> MAEVLRTLAGKPKCHALRPMILFLIMLVLVLFGYGVLSPRSLMPGSLERGFCMAVREPDHLQRVSLPRMVYPQPKVLTPCRKDVLVVTPWLAPIVWEGTFNIDILNEQFRLQNTTIGLTVFAIKKYVAFLKLFLETAEKHFMVGHRVHYYVFTDQPAAVPRVTLGTGRQLSVLEVRAYKRWQDVSMRRMEMISDFCERRFLSEVDYLVCVDVDMEFRDHVGVEILTPLFGTLHPGFYGSSREAFTYERRPQSQAYIPKDEGDFYYGGAFFGGSVQEV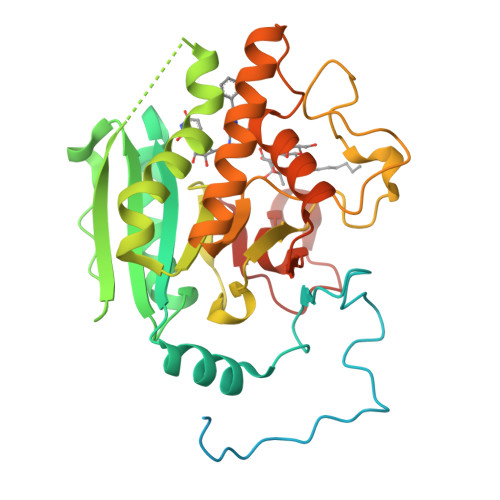QRLTRACHQAMMVDQANGIEAVWHDESHLNKYLLRHKPTKVLSPEYLWDQQLLGWPAVLRKLRFTAVPKNHQAVRNP> GSSST;> GLGQMLESMIDNTVRETVGAATSRDALPNTEASGPTHSKEIPALTAVETGATNPLVPSDTVQTRHVVQHRSRSESSIESFFARGACVTIMTVDNSASTTNKDKLFAVWKITYKDTVQLRRKLEFFTYSRFDMELTFVVTANFTETNNGHALNQVYQIMYIPPGAPVPEKWDDYTWQTSSNPSIFYTYGTAPARISVPYVGISNAYSHFYDGFSKVPLKDQSAALGDSLYGAASLNDFGILAVRVVNDHNPTKVTSKIRVYLKPKHIRVWCPRPPRAVAYYGPGVDYKDGTLTPLSTKDLTTY;> SPNIEACGYSDRVLQLTLGNSTITTQEAANSVVAYGRWPEYLRDSEANPVDQPTEPDVAACRFYTLDTVSWTKESRGWWWKLPDA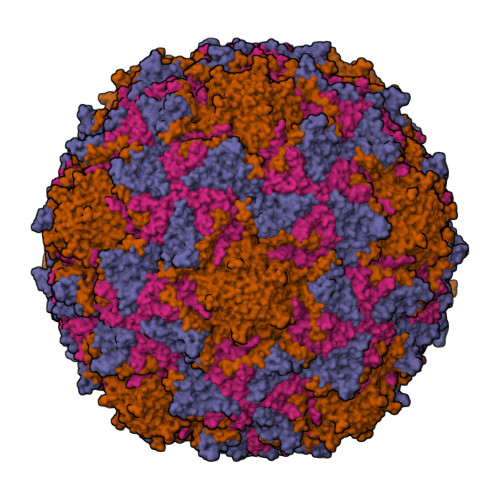LRDMGLFGQNMYYHYLGRSGYTVHVQCNASKFHQGALGVFAVPEMCLAGDSNTTTMHTSYQNANPGEKGGTFTGTFTPDNNQTSPARRFCPVDYLLGNGTLLGNAFVFPHQIINLRTNNCATLVLPYVNSLSIDSMVKHNNWGIAILPLAPLNFASESSPEIPITLTIAPMCCEFNGLRNITLPRLQ;> GLPVMNTPGSNQYLTADNFQSPCALPEFDVTPPIDIPGEVKNMMELAEIDTMIPFDLSATKKNTMEMYRVRLSDKPHTDDPILCLSLSPASDPRLSHTMLGEILNYYTHWAGSLKFTFLFCGSMMATGKLLVSYAPPGADPPKKRKEAMLGTHVIWDIGLQSSCTMVVPWISNTTYRQTIDDSFTEGGYISVFYQTRIVVPLSTPREMDILGFVSACNDFSVRLLRDTTHIEQKALAQ;> GAQVSSQKVGAHENSNRAYGGSTINYTTINYYRDSASNAASKQDFSQDPSKFTEPIKDVLIKTAPMLN Mammalian lactate dehydrogenase D (LDHD) catalyzes the oxidation of D-lactate to pyruvate. We demonstrate that mLDHD is an Mn2+-dependent general dehydrogenase which exhibits catalytic activity for D-lactate and other D-2-hydroxyacids containing hydrophobic moieties, but no activity for their L-isomers or D-2-hydroxyacids containing hydrophilic moieties. Similar to other members of the VAO/PCMH flavoprotein family, mLDHD consists of an FAD-binding domain, a substrate-binding domain and a C-terminal domain. The substrate-binding site contains a positively charged pocket to bind the common glycolate moiety and a hydrophobic pocket with some elasticity to bind the varied hydrophobic moieties of substrates.

Crystallization experiments show that soaking of the mLDHDFAD crystals in crystallization solution supplemented with the substrates and MnCl2 often yields the product-bound or mixed substrate/product-bound structures. Thus, we prepared the loss-of-function H405A mutant mLDHD (mLDHDH405A), and determined the crystal structures of the mLDHDH405A mutant in FAD-bound form and in complexes with FAD and various substrates (D-lactate, D-2-hydroxybutyrate, D-2-hydroxyvalerate, D-2-hydroxyhexanoic acid, D-2-hydroxyoctanoate, D-2-hydroxyisovalerate, D-2-hydroxyisocaproate, and D-2-hydroxy-3-methylvalerate) at high resolutions (1.31–1.75 Å). In the substrate-bound mLDHD and mLDHDH405A structures, all the substrates are clearly defined in the electron density maps; however, Mn2+ is only identified at the active site in the WT structure, but not in the mutant structures due to the mutation of the metal-coordinating His405. Although the DL-isomer mixtures of some substrates (DL-2-hydroxyvalerate, DL-2-hydroxyhexanoate, DL-2-hydroxyoctanoate, DL-2-hydroxyisocaproate, and DL-2-hydroxy-3-methylvalerate) were used in the crystallization experiments, only the D-isomers bind to the active site, further confirming that mLDHD has high stereo-selectivity for the D-isomers over the L-isomers. Comparison of the D-lactate-bound and other substrate-bound mLDHDH405A structures also reveals no major conformational changes for the residues at the substrate-binding subsite A, and the other substrates bind to the same site and the C1-carboxyl and C2-hydroxyl groups of substrates maintain similar hydrogen-bonding interactions with the surrounding residues as D-lactate. However, along with the increase of the size of the hydrophobic moiety of substrate, the key residues composing the substrate-binding subsite B undergo conformational changes to varied extents to accommodate the larger hydrophobic moiety. Concurrently, the larger hydrophobic moiety of substrate makes more hydrophobic interactions with the surrounding residues.

> WSHPQFEKGSQGGLSQDFVEALKAVVGSPHVSTASAVREQHGHDESMHRCQPPDAVVWPQNVDQVSRVASLCYNQGVPIIPFGTGTGVEGGVCAVQGGVCINLTHMDQITELNTEDFSVVVEPGVTRKALNTHLRDSGLWFPVDPGADASLCGMAATGASGTNAVRYGTMRDNVINLEVVLPDGRLLHTAGRGRHYRKSAAGYNLTGLFVGSEGTLGIITSTTLRLHPAPEATVAATCAFPSVQAAVDSTVQILQAAVPVARIEFLDDVMMDACNRHSKLNCPVAPTLFLEFHGSQQTLAEQLQRTEAITQDNGGSHFSWAKEAEKRNELWAARHNAWYAALALSPGSKAYSTDVCVPISRLPEILVETKEEIKASKLTGAIVGHVGDGNFACILLVDPDDAEEQRRVKAFAENLGRRALALGGTCTGEHGIGLGKRQLLQEEVGPVGVETMRQLKNTLDPRGLMNPGKVL>[2x]MAGRWNLEGCTALVTGGSRGIGYGIVEELASLGASVYTCSRNQKELNDCLTQWRSKGFKVEASVCDLSSRSERQELMNTVANHFHGKLNILVNNAGIVIYKEAKDYTVEDYSLIMSINFEAAYHLSVLAH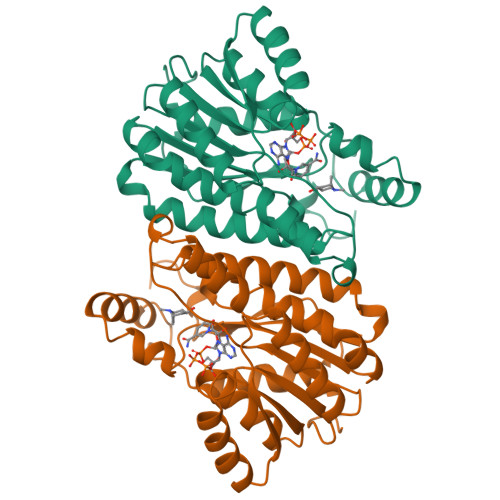PFLKASERGNVVFISSVSGALAVPYEAVYGATKGAMDQLTRCLAFEWAKDNIRVNGVGPGVIATSLVEMTIQDPEQKENLNKLIDRCALRRMGEPKELAAMVAFLCFPAASYVTGQIIYVDGGLMANCGF> MRVKHAVVLLMLISPLSWAGTMTFQFRNPNFGGNPNNGAFLLNSAQAQNS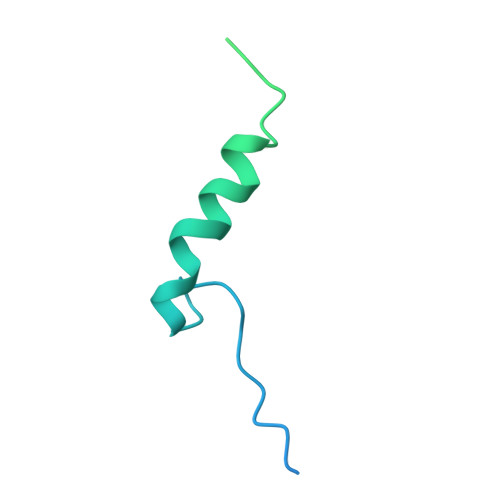YKDPSYNDDFGIETPSALDNFTQAIQSQILGGLLSNINTGKPGRMVTNDYIVDIANRDGQLQLNVTDRKTGQTSTIQVSGLQNNSTDF> AGAGAAAA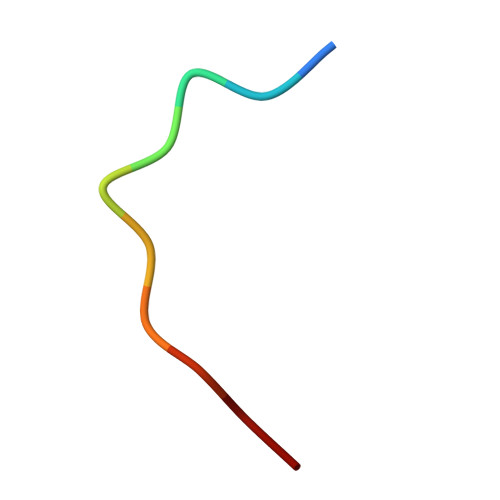AA>SNAMNYFELFGLPIQFELDGSLLSSQFRALQKRFHPDNFATASERDRLMAVQQAAQINDAYQTLKDPLRRAEYLLSLQGIEMNAEQQTLQDP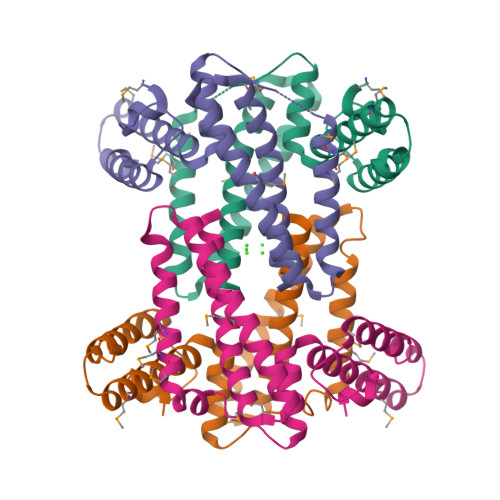MFLMEQMELREELESVTACADPEAALVAFDTKVTAMQRHYLAQLQGQLAQSEWLAAADQIRKLKFIAKLKNEVERVEDQLLG[4x]>[3x]MGAMIVKEVYETAEKIKSMEIRG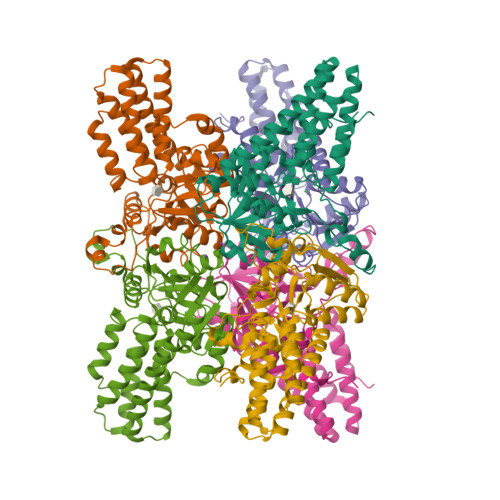AGRIARAAAQALMIQAEKSKAKEPEELWNELKVASKILYNTRPTAVSLPNALRYVMHRVKAAYLGGADLETLRFTAINSAKEFIYNSEKAIERIGEIGAKRIEDGDIIMTHSHSKAAISVMKKAFEQGKNIKVIVTETRPKWQGKITAKELASYGIPVIYIVDSAARHYMKMTDKVVMGADSITANGAVINKIGTSLIALTAKEHRVWVMIAAETYKFHPATMLGQLVEIEMRDPTEVIPEEELRTWPKNIEVWNPAFDVTPPEYIDVIITERGIIPPYAAIDILKEEFGWALKYKEPWED> RSQRLVFNRPFLMFIVDNNILFL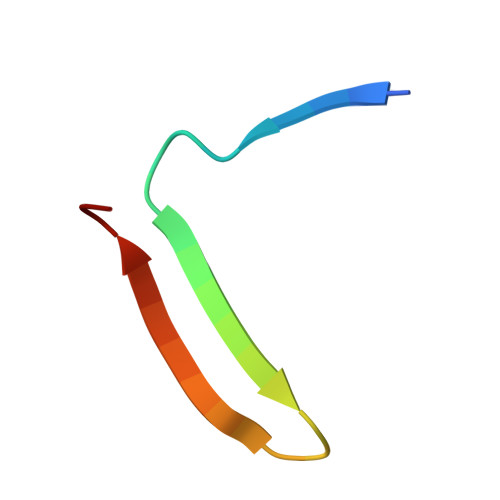GKVNRP>MTSILTNNSAMAALSGVRSISSSMEDTQSRISSGLRVGSASDNAAYWSIATTMRSDNQALSAVQDALGLGAAKVDTAYSGMESAIEVVKEIKAKLVAATEDGVDKAKIQEEITQLKDQLTSIADAASFSGENWLQADLSGGAVTKSVVGSFVRDGSGSVAVKKVDYSLNANSVLFDTVGDTGILDKVYNVSQASVTLTVNTNGVESQHTVAAYSLESLTEAGAEFQGNYALQGGNSYVKVENVWVRAETAATGATGQEIAATTTAAGTI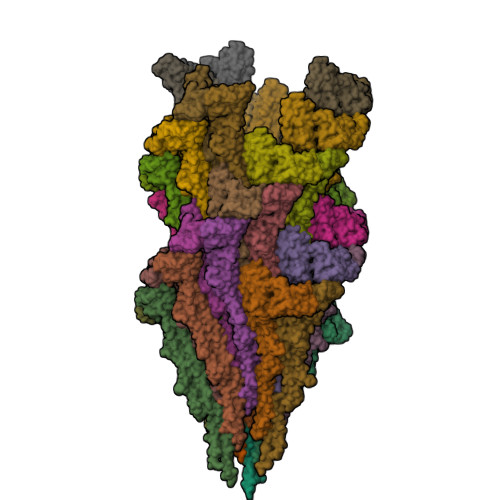TADSWVVDVGNAPAANVSAGQSVANINIVGMGAAALDALISGVDAALTDMTSAAASLGSISSRIDLQSEFVNKLSDSIESGVGRLVDADMNEESTRLKALQTQQQLAIQALSIANSDSQNVLSLFR[42x]5-[2-[(3,4-dichlorophenyl)carbonylamino]ethyl]-~{N}-oxidanyl-1,2-oxazole-3-carboxamide 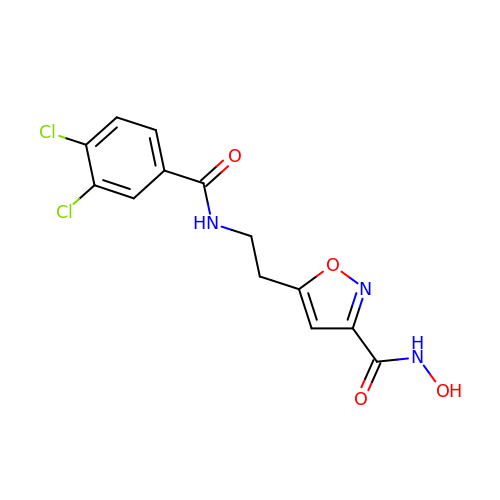| C13 H11 Cl2 N3 O4 | JFGOILLZIAIYGA-UHFFFAOYSA-N> ESLYQSKYEELQITAGR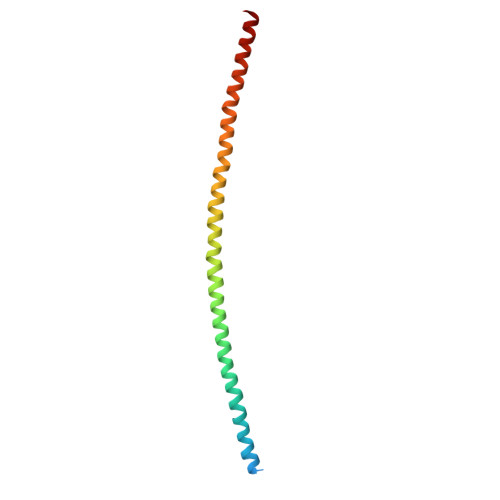HGDSVRNSKIEISELNRVIQRLRSEIDNVKKQISNLQQSISDAEQRGENALKDAKNKLNDLEDALQQAKEDLARLLRDYQELMNTKLALDLEIATYRTLLEGE> MGHHHHHHHHHHSSGHIDDDDKMKVLTELQKQIFTIVKKENGKPIPPGIVVRMMENSPNFPGKHLIYRAIDDLLDWAILRKAGGVTNQLLVNYEPAEPLLDKKLQGILTLGNKNSGFIRSLDDDKTVYYVHYSNLTGALDGDLVEFCKLDKPQFGDKFDAAVITILKRARILYAGNFLVDQNEFALEYKIVADNPRFYLTMIVNPDSIPNNLASNTKIAFQIDEYDPDNNLCKVSVQQVLGNNDDPLINIKAIMLDNSIVFETNDVVEQHANKLSFDTEEQHKAYRQDLTDLAFVTVDPTTSKDLDDAIYVKTIPTGFVLYVAIADVAHYVNRNSEIDIEAKHKTSSIYLPGHYVVPMLPEQLSNQLCSLNPAQKR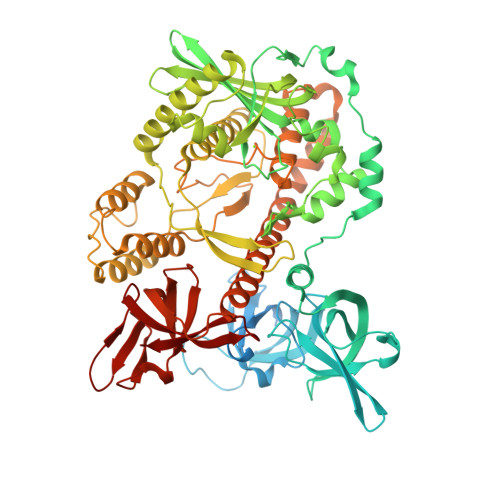YVVVCEISFDNQGRIKTNKLYPATIISKNRFSYDQVNKWLNNKSELNCDETVINSLKAAFTLSDLIQAQRQKRGTIDLSHKETEIVVDEHYFPIKINFLVHDKAETMIENLMVVANETVAWVLTNNKIALPYRVHPRPSKKKLQSLIETVGELNITKPQFNLDTVTSSQIASWLNENKDNPSYEIFVILLLRTLGKAFYSVNPLMHFSIGSNHYTHFTSPIRRYIDLTIHRLLWMHLFTPDQFTDNERDQLKQELEKIADTVNDTEIKIINCERNANDYLTTLLLSKQIGKTFSGFISAITSFGIFMRMDENNFDGLIKITTIPDDFFIFEKEKMVLKGRKTNKVYKIGDRLEAKLSEIDFIQKRAILTLI>[2x]ISEFGSEPIDPS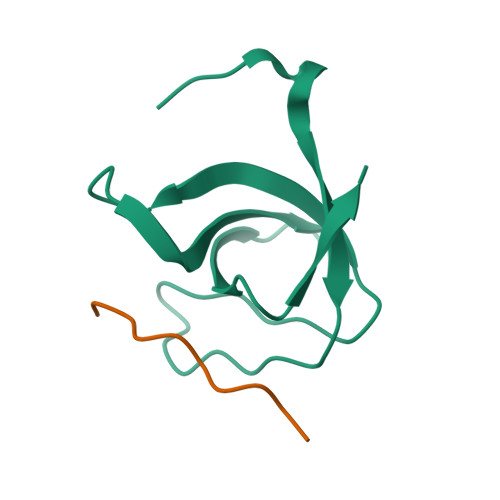KLEFARALYDFVPENPEMEVALKKGDLMAILSKKDPLGRDSDWWKVRTKNGNIGYIPYNYIEIIKRRKKIEHVDDETRTH;>[2x]EAMPPTLPHRDWKD>MGSSHHHHHHSSGPQQGLRSNSDDAEKPVVPVPTGDVAIYTTTSSLTRDLTRDAVNFSPKDNLAPTTITLNPAEQYQTMDGFGAAITGSTCYNLLLMKPADRHAFLTETFSDKDGFGFSYIRISIGCSDFSLSEYTCCDTKGIENFALQSEEKDYILPILKEILAINPSIKVIAAPWTCPKWMKVKSLTDRTPLDSWTNGQLNPDYYQDYATYFVKWIQAFKAEGIDIYAVTPQNEPLNRGNSASLYMEWEEQRDFVKTALGPQMKAAGLSTKIYAFDHNYNYDNIESQKNYPGKIYEDAAASQYLAGAAYHNYGGNREELLNIHQAYPEKELLFTETSIGTWNSGRDLSKRLMEDMEEVALGTINNWCKGVIVWNLMLDNDRGPNREGGCQTCYGAVDINNSDYKTIIRNSHYYIIAHLSSVVKPGAVRIATTGYTDNGITCSAFENTDGTYAFVL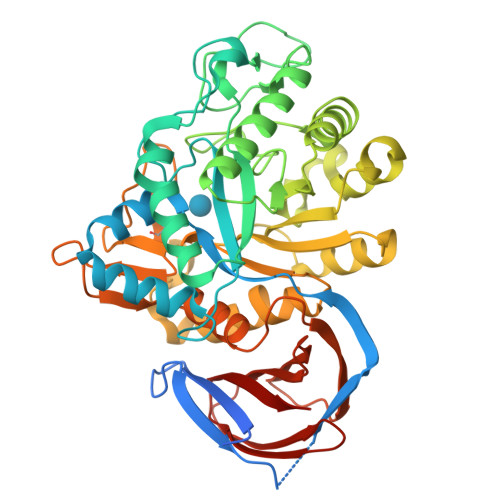INNNEKSKKITVSDGQRHFAYDVPGKSVTSYRWAKSK[3x]> MDYKDDDDKMSAKKIVLKSSDGESFEVEEAVALESQTIAHMVEDDCVDNGVPLPNVTSKILAKVIEYCKRHVEAAASKAEAVEGAATSDDDLKAWDADFMKIDQATLFELILAANYLNIKNLLDLTCQTVADMIKGKTPEEIRTTF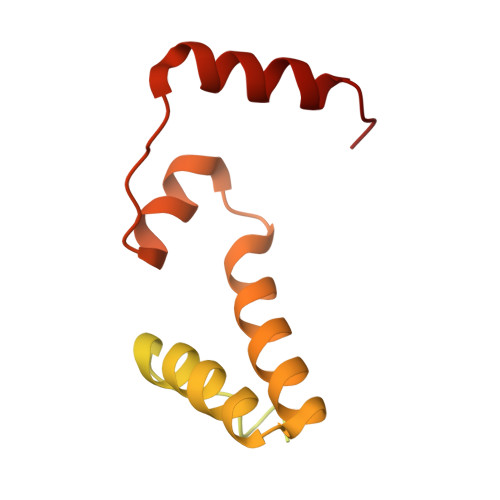NIKNDFTPEEEEEVRRENQWAFE>MHTLYAPGGYDIMGYLIQIMNRPNPQVELGPVDTSCALILCDLKQKDTPIVYASEAFLYMTGYSNAEVLGRNCRFLQSPDGMVK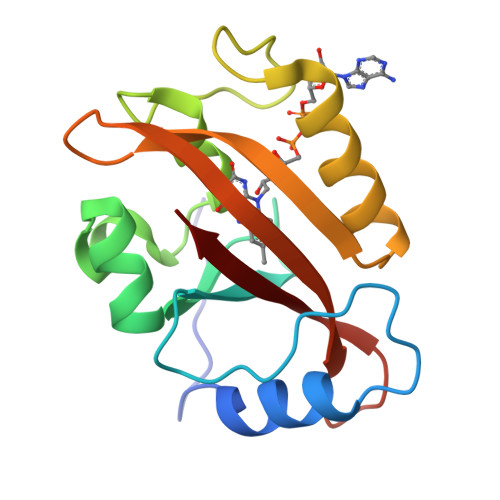PKSTRKYVDSNTINTMRKAIDRNAEVQVEVVNFKKNGQRFVNFLTMIPVRDETGEYRYSMGFQCE[2x]> MATFTTEQAGYQMQAILQVIGYDLLIVVTGGTNPHIG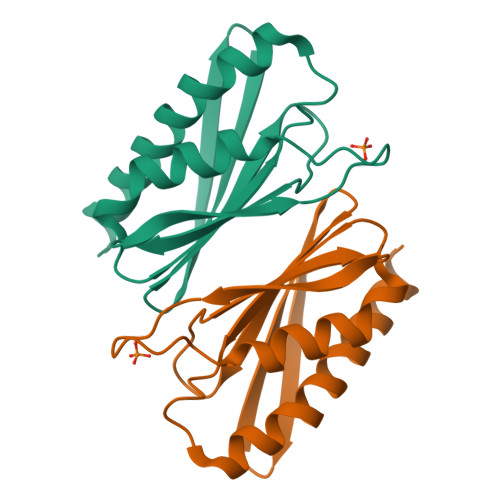DVTTLTASTVPETVKFPSHDGRFHKDNFISERMAKRIQRYLAGSCTITAGIHVNQITKAQIAAAAPMTDDLSRQIISWLQAHPVQAEKPEYYGQDEQPR> SASPQEQDQDRRKDWGHVELLEVLQARVRQLQAESVSEVVVNRVDVARLPECGSGDGSLQPPRKVQMGAKDATPVPCGRWAKILEKDKRTQQMRMQRLKAKLQMPFQSGEFKALTRRLQVEPRLLSKQMAGCLEDCTRQAPESPWEEQLARLLQEAPGKLSLDVEQAPSGQHSQAQLSGQQQRLLAFFKCCLLTDQLPLAHHLLVVHHGQRQKRKLLTLDMYNAVMLGWARQGAFKELVYVLFMVKDAGLTPDLLSYAAALQCMGRQDQDAGTIERCLEQMSQEGLKLQALFTAVLLSEEDRATVLKAVHKVKPTFSLPPQLPPPVNTSKLLRDVYAKDGRVSYPKLHLPLKTLQCLFEKQLHMELASRVCVVSVEKPTLPSKEVKHARKTLKTLRDQWEKALCRALRETKNRLEREVYEGRFSLYPFLCLLDEREVVRMLLQVLQALPAQGESFTTLARELSARTFSRHVVQRQRVSGQVQALQNHYRKYLCLLASDAEVPEPCLPRQYWEELGAPEALREQPWPLPVQMELGKLLAEMLVQATQMPCSLDKPHRSSRLVPVLYHVYSFRNVQQIGILKPHPAYVQLLEKAAEPTLTFEAVDVPMLCPPLPWTSPHSGAFLLSPTKLMRTVEGATQHQELLETCPPTALHGALDALTQLGNCAWRVNGRVLDLVLQLFQAKGCPQLGVPAPPSEAPQPPEAHLPHSAAPARKAELRRELAHCQKVAREMHSLRAEALYRLSLAQHLRDRVFWLPHNMDFRGRTYPCPPHFNHLGSDVARALLEFAQGRPLGPHGLDWLKIHLVNLTGLKKREPLRKRLAFAEEVMDDILDSADQPLTGRKWWMGAEEPWQTLACCMEVANAVRASDPAAYVSHLPVHQDGSCNGLQHYAALGRDSVGAASVNLEPSDVPQDVYSGVAAQVEVFRRQDAQRGMRVAQ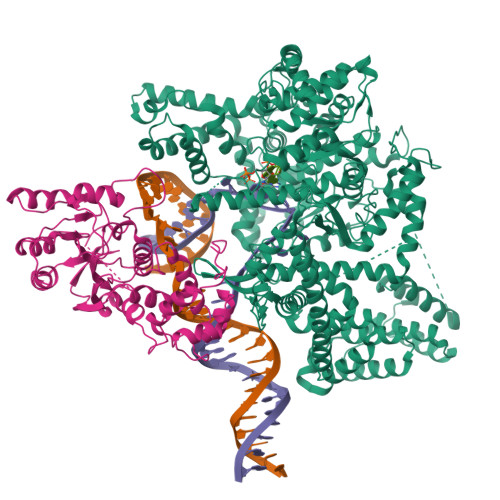VLEGFITRKVVKQTVMTVVYGVTRYGGRLQIEKRLRELSDFPQEFVWEASHYLVRQVFKSLQEMFSGTRAIQHWLTESARLISHMGSVVEWVTPLGVPVIQPYRLDSKVKQIGGGIQSITYTHNGDISRKPNTRKQKNGFPPNFIHSLDSSHMMLTALHCYRKGLTFVSVHDCYWTHAADVSVMNQVCREQFVRLHSEPILQDLSRFLVKRFCSEPQKILEASQLKETLQAVPKPGAFDLEQVKRSTYFFS;> PPRKASKASLDFKRYVTDRRLAETLAQIYLGKPSRPPHLLLECNPGPGILTQALLEAGAKVVALESDKTFIPHLESLGKNLDGKLRVIHCDFFKLDPRSGGVIKPPAMSSRGLFKNLGIEAVPWTADIPLKVVGMFPSRGEKRALWKLAYDLYSCTSIYKFGRIEVNMFIGEKEFQKLMADPGNPDLYHVLSVIWQLACEIKVLHMEPWSSFDIYTRKGPLENPKRRELLDQLQQKLYLIQMIPRQNLFTKNLTPMNYNIFFHLLKHCFGRRSATVIDHLRSLTPLDARDILMQIGKQEDEKVVNMHPQDFKTLFETIERSKDCAYKWLYDETLEDR>[16x]ANSHHHHHHGKLTSDFDNPRWIGRHKHMFNFLDVNHNGKISLDEMVYKASDIVINNLGATPEQAKRHKDAVEAFFGGAGMKYGVETDWPAYIEGWKKLATDELEKYAKNEPTLIRIWGDALFDIVDKDQNGAITLDEWKAYTKAAGIIQSSEDCEETFRVCDIDESGQLDVDEMTRQHLGFWYTMDPACEKLYGGAVP

The Ca2+-binding photoprotein aequorin is a complex of apoAequorin (apoprotein) and (S)-2-peroxycoelenterazine. apoAequorin, which consists of 189 amino acid residues, can be regenerated to aequorin by incubation with coelenterazine and O2, both in vivo and in vitro. The chiral deaza-analogs of (S)-daCTZ and (S)-HM-daCTZ selectively inhibited the regeneration step to aequorin by binding the catalytic site of coelenterazine in the apoAequorin molecule. The crystal structures of the apoAequorin complexes with (S)-daCTZ and (S)-HM-daCTZ were determined, suggesting that the hydroxy moiety at the C6-hydroxyphenyl group and the carbonyl moiety of the imidazopyrazinone ring in coelenterazine are essential to bind the apoAequorin molecule through hydrogen bonding.

As the deaza-analogs of (S)-daCTZ and (S)-HM-daCTZ were regarded as coelenterazine and (S)-2-peroxycoelenterazine, respectively, (S)-daCTZ could be used as a probe to determine the recognition residues of apoAequorin and (S)-HM-daCTZ could be applied to confirm the binding environment of (S)-2-peroxycoelenterazine in apoAequorin, as previously reported. Moreover, the deaza-analog of (R)-daCTZ and (S)-daCTZ for coelenterazine inhibited the aequorin regeneration and the inhibition with (S)-daCTZ was stronger than that with (R)-daCTZ. The strong inhibition of (S)-daCTZ and (S)-HM-daCTZ on aequorin regeneration indicate that the deaza-analogs can generate a stable complex with apoAequorin. The asymmetric unit of the crystal contained two molecules of the deaza-CTZ analog/apoAequorin complex and formed 16 molecules of the deaza-CTZ analog/apoAequorin complex, similar to the case of cf3-aequorin. In the apoAequorin/(S)-daCTZ complex, the p-hydroxy moiety at the C6-hydroxyphenyl group was stabilized by the amino acid triad of His16, Tyr82, and Trp86, and the C3-carbonyl group of the indanone structure in (S)-daCTZ interacted with His169 in hydrogen-bonding distances. The p-hydroxy moiety at the C2-hydroxyphenyl group was stabilized with I105 and T166 through a water molecule, identical to that of native aequorin. Thus, apoAequorin can recognize the p-hydroxy moiety at the C6-hydroxyphenyl group and the C3-carbonyl moiety in coelenterazine to bind coelenterazine. Similarly, the regeneration to aequorin from the apoAequorin/(S)-daCTZ complex by incubation with coelenterazine was performed, and the results revealed that the deaza-analog binds non-covalently to apoAequorin, enabling the replacement with coelenterazine to convert active aequorin.> SMENKNLNYILGLDLGIASVGWAVVEIDEKENPLRLIDVGVRTFERAEVPKTGESLALSRRLARSARRLTQRRVARLKKAKRLLKSENILLSTDERLPHQVWQLRVEGLDHKLERQEWAAVLLHLIKHRGYLSQRKNESKSENKELGALLSGVDNNHKLLQQATYRSPAELAVKKFEVEEGHIRNQQGAYTHTFSRLDLLAEMELLFSRQQHFGNPFASEKLLENLTALLMWQKPALSGEAILKMLGKCTFEDEYKAAKNTYSAERFVWITKLNNLRIQENGLERALNDNERLALMEQPYDKNRLFYSQVRSILKLSDEAIFKGLRYSGEDKKAIETKAVLMEMKAYHQIRKVLEGNNLKAEWAELKANPTLLDEIGTAFSLYKTDEDISAYLAGKLSQPVLNALLENLSFDKFIQLSLKALYKLLPLMQQGLRYDEACREIYGDHYGKKTEENHHFLPQIPADEIRNPVVLRTLTQARKVINGVVRLYGSPARIHIETGREVGKSYKDRRELEKRQEENRKQRENAIKEFKEYFPHFAGEPKAKDILKMRLYKQQNAKCLYSGKPIELHRLLEKGYVEVDHALPFSRTWDDSFNNKVLVLANENQNKGNLTPFEWLDGKHNSERWRAFKALVETSAFPYAKKQRILSQKLDEKGFIERNLNDTRYVARFLCNFIADNMHLTGEGKRKVFASNGQITALLRSRWGLAKSREDNDRHHALDAVVVACSTVAMQQKITRFVRFEAGDVFTGERIDRETGEIIPLHFPTPWQFFKQEVEIRIFSDNPKLELENRLPDRPQANHEFVQPLFVSRMPTRKMTGQGHMETVKSAKRLNEGISVIKMPLTKLKLKDLELMVNREREKDLYDTLKARLEAFNDDPAKAFAEPFIKKGGA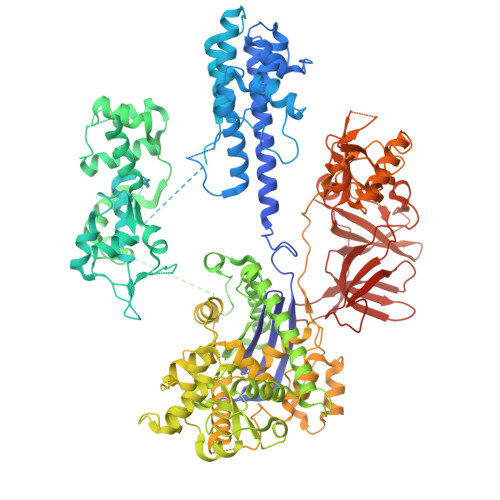IVKSVRVEQIQKSGVLVREGNGVADNASMVRVDVFTKGGKYFLVPIYTWQVAKGILPNKAATQYKDEEDWEVMDNSATFKFSLHPNDLVKLVTKKKTILGYFNGLNRATGNIDIKEHDLDKSKGKQGIFEGVGIKLALSFEKYQVDELGKNIRLCKPSKRQPVR> GSGS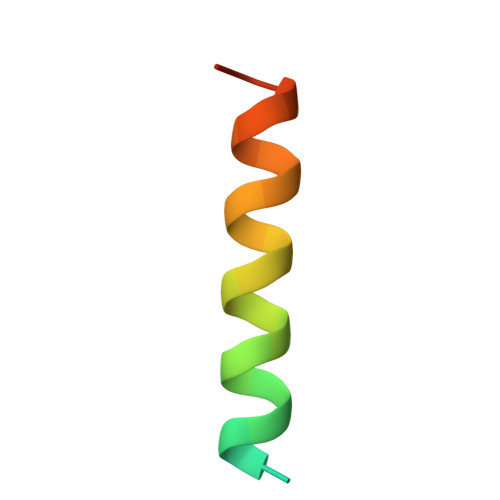GSGSGSSATRELDELMASLSDFKMQGLE SWI/SNF is the prototype chromatin remodeling complex and regulates the expression of 5% genes in yeast. Within SWI/SNF, Snf2 functions as the ATP-dependent motor that drives the fundamental DNA translocation reaction underlying chromatin remodeling, whereas many of the auxiliary subunits target the enzyme to specific loci of the genome. To understand the mechanism of nucleosome recognition, we report the cryo-EM structure of the yeast SWI/SNF complex in complex with the mononucleosome. Based on the specific biological activities involved, the SWI/SNF complex is delineated into three functional modules: the motor module, the actin-related protein (ARP) module, and SRM.

Most of the auxiliary subunits are assembled into the SRM, which is further delineated into two lobes, the DNA-binding lobe (DBL), and the histone-binding lobe (HBL). These auxiliary subunits recognize different features of the DNA and histone components of the nucleosome, and collectively provide the structural basis for chromatin targeting of the complex. DBL of SWI/SNF is composed of multiple elements, including Snf6, the N-termini of Swi1 and Snf5, and Snf12, which directly or indirectly bind to the DNA. The N-termini of Swi1 and Snf5 interact with each other, which may bind to the DNA of nucleosome either through the ARID domain directly, or indirectly through transcription coactivators, providing the structural basis for their cooperation in SWI/SNF targeting. HBL contains two important elements for histone binding, Snf5 and Taf14. A fragment of the C-terminal tail was found, which folded back and sandwiched between Swi3 and Swp82 at the HBL. Intriguingly, at the periphery of the DBL, we identified an IgG-fold domain of Snf12. Because the SWIB domain inserts into the β6–β7 loop, the IgG-fold is barely detectable at the sequence level. Structural comparison indicated that this IgG-fold domain shows a strong analogy to the YEATS domain of TAF14. This YEATS-like domain is ~9 nm away from the exit DNA without any steric hindrance, which would allow binding to transcription factors in a manner similar to the SWIB domain.

> LQDQYKEGIKVVDIDDPDMMVDSFTMPNISHSNIDYQTLLANSDHAKFTIEPGVLPVGIDTHTATDIYQTLIALNLDTTVNDCLDKLLNDECTESTRENALYDYYALQLLPLQKAVRGHVLQFEWHQNSLLTNTHPNFLSKIRNINVQDALLTNQLYKNHELLKLERKKTEAVARLKSMNKSAINQYNRRQDKKNKRLKFGHRLIATHTNLERDEQKRAEKKAKERLQALKANDEEAYIKLLDQTKDTRITHLLRQTNAFLDSLTRAVKDQQKYTKEMIDSHIKEASEEVDDLSMVPKMKDEEYDDDDDNSNVDYYNVAHRIKEDIKKQPSILVGGTLKDYQIKGLQWMVSLFNNHLNGILADEMGLGKTIQTISLLTYLYEMKNIRGPYLVIVPLSTLSNWSSEFAKWAPTLRTISFKGSPNERKAKQAKIRAGEFDVVLTTFEYIIKERALLSKVKWVHMIIDEGHRMKNAQSKLSLTLNTHYHADYRLILTGTPLQNNLPELWALLNFVLPKIFNSVKSFDEWFNTPFANTGGQDKIELSEEETLLVIRRLHKVLRPFLLRRLKKDVEKELPDKVEKVVKCKMSALQQIMYQQMLKYRRLFIGDQNNKKMVGLRGFNNQIMQLKKICNHPFVFEEVEDQINPTRETNDDIWRVAGKFELLDRILPKLKATGHRVLIFFQMTQIMDIMEDFLRYINIKYLRLDGHTKSDERSELLRLFNAPDSEYLCFILSTRAGGLGLNLQTADTVIIFDTDWNPHQDLQAQDRAHRIGQKNEVRILRLITTNSVEEVILERAYKKLDIDGKVIQAGKFDNKSTSEEQEALLRSLLDAEEERRKKRESGVEEEEELKDSEINEILARNDEEMAVLTRMDEDRSKKEEELGVKSRLLEKSELPDIYSRDIGAELKREESESAAVYNGRGARERKTATYNDNMSEEQWLRQFEVSDDEKNDKQARKQRTKKEDKSEAIDGGGSGGHHHHHH;> SNQLISNYAASNSMDRSSSASNEFVPNTSDNNNNSNNHNMRNNSNNKTSNNNNVTAVPAATPANTNNSTSNANTVFSERAAMFAALQQKQQQRFQALQQQQQQQQNQQQQNQQPQQQQQQQQNPKFLQSQRQQQQRSILQSLNPALQEKISTELNNKQYELFMKSLIENCKKRNMPLQSIPEIGNRKINLFYLYMLVQKFGGADQVTRTQQWSMVAQRLQISDYQQLESIYFRILLPYERHMISQEGIKETQAKRIFLQQFLQELLKKVQQQQQAAALANANNNINSASSAPTPAAPGASVPATAAPGTEAGIVPVSANTPKSLNSNININVNNNNIGQQQVKKPRKQRVKKKTKKELELERKEREDFQKRQQKLLEDQQRQQKLLLETKLRQQYEIELKKLPKVYKRSIVRNYKPLINRLKHYNGYDINYISKIGEKIDSNKPIFLFAPELGAINLHALSMSLQSKNLGEINTALNTLLVTSADSNLKISLVKYPELLDSLAILGMNLLSNLSQNVVPYHRNTSDYYYEDAGSNQYYVTQHDKMVDKIFEKVNNNATLTPNDSNDEKVTILVDSLTGNQLPTPTPTEMEPDLDTECFISMQSTSPAVKQWDLLPEPIRFLPNQFPLKIHRTPYLTSLKKIKDEIDDPFTKINTRGAEDPKVLINDQLSTISMILRNISFSDNNSRIMSRNFYLKRFISDLLWLVLIHPENFTCNRKILNFKKDLVIVLSNISHLLEIASSIDCLLILILVISFGQPKLNPMASSSSFGSESLTFNEFQLQWGKYQTFGVDILAKLFSLEKPNLNYFKSILLNKNTGNNLYDRNSNNNHKDKKLLRRLLNLYNDNNKNNNNRHNLLNDVVSFLFSAIPLQQVLSQSADPSLLIDQFSPVISQSLTSILVIVQKILPLSNEVFEISENNSDSNSNNNGNKDSSFNFNKNLPFVWLSSEENIGSGLLKLSEIILNINNSTSKNTLLQQQNYSKVLLPSINISCVQLIKCLVEKSICFENCLNNDPEILKKIASIPNLFPTDLEIFQLFTNPSVDIQIINQYQLLYNLKNDILTNLEGGSGGWSHPQFEKWSHPQFEKWSHPQFEK;> MNNQPQGTNSVPNSIGNIFSNIGTPSFNMAQIPQQLYQSLTPQQLQMIQQRHQQLLRSRLQQQQQQQQQTSPPPQTHQSPPPPPQQSQPIANQSATSTPPPPPAPHNLHPQIGQVPLAPAPINLPPQIAQLPLATQQQVLNKLRQQAIAKNNPQVVNAITVAQQQVQRQIEQQKGQQTAQTQLEQQRQLLVQQQQQQQLRNQIQRQQQQQFRHHVQIQQQQQKQQQQQQQHQQQQQQQQQQQQQQQQQQQQQQQQQQQQQQQQQQQQQGQIPQSQQVPQVRSMSGQPPTNVQPTIGQLPQLPKLNLPKYQTIQYDPPETKLPYPTYWSDKKADTDTLLYEQIIQRDKINKYSLIRETNGYDPFSIYGFSNKEYISRLWHTLKYYQDLKNTRMKSITSTSQKIPSASIWGNGYSGYGNGITNTTTRVIPQVEVGNRKHYLEDKLKVYKQAMNETSEQLVPIRLEFDQDRDRFFLRDTLLWNKNDKLIKIEDFVDDMLRDYRFEDATREQHIDTICQSIQEQIQEFQGNPYIELNQDRLGGDDLRIRIKLDIVVGQNQLIDQFEWDISNSDNCPEEFAESMCQELELPGEFVTAIAHSIREQVHMYHKSLALLGYNFDGSAIEDDDIRSRMLPTITLDDVYRPAAESKIFTPNLLQISAAELERLDKDKDRDTRRKRRQGRSNRRGMLALSGTSASNTSMNGVHNTVAAGNASSLPPGEILLPDIADIPRTFRTPVPSTLMPGGVDVGPSVESYELRNTTTYKSRPDRPKPVSPPCYIIDHIPGHSLLLSIKLPGKVNTKEEFAAAPNDTSSGTNAMLPSPESLKTKLNSNIRAGVTIPSIPNPIANHTVTNSPNPTLQPVIPGGAASKSVPTPSLPIAPPVAPHDSEATLLTNSNNGSSNNNTQNTGGSGGDYKDDDDK;>[2x]MENTLGEGSTVNASVDVDQHGNDNNSDSNANAAVAGVANTDTAGEESQQQDESLKDEATVPNTRDAESEAITVTAKQQPTMQANKLDSQETPSTEESRAQNVFGQDNEDSDNLFGETESSVSNNEANTPSIPTNPVDNENNKPAIKEDSTIQDSNGDVKNMEDVKIQKEEEPENNTVIEGVKEESQPDENTKEMDEVEEDDEDDDQPMISPDNSIFGDTKSESKQLGNTSSVANTPSEIPDAHKAEQEDIIEKTESVDKKVDSGEERNEQEREIMNDHSKSANPKKTTITRVEPETFEIPQAHEIVIPSYSKWFNLEKIHSIEVQSLPEFFTNRIPSKTPEVYMRYRNFMVNSYRLNPNEYFSVTTARRNVSGDAAALFRLHKFLTKWGLINYQVDSKLLPKNIEPPLTSQYSTRHDAPRGLFPFESYKPSVQLPDMAKLKKMMNTSDSESTLYKYLKESKRKYDEITHPPSTTDDENGDKNDNGGKMNNEVSTSTSMTGDANLLEEGETSRPLKKVKILEQIDENWSKEDLQKLLKGIQEFGADWYKVAKNVGNKSPEQCILRFLQLPIEDKFLYGDGNGKGDNDNGLGPLKYAPHLPFSKSENPVLSTIAFLVGLVNPKTVQSMTQRAIQSAESIKSQKEEISDQKPIEHIKEGSEIAISSLGYRSHIFATNEERQMNFLTNELIRLQMEKLDAKLNHLKKLEKFMELERKTLERQQENLLIQRLNFNQNSSKIVNVLSKCLNLISDSNINNSSVAEKEEIRSQIDHFKSMLSKPETLSIGKNPFNKPNIETGENHNGQSISNENDVKPISIEAPQFYRYWSAGGSGGHHHHHH;> MSKVMKPSNGKGSRKSSKAATPDTKNFFHAKKKDPVNQDKANNASQITPTVPHSHPSDMVIPDHLAELIPELYSFQQLVDSEKRLDHFIHLRNLHMKRMVAQWERSKLSQEFLYPHLNFPNVKFLRIFISNVSENQPWQMDTNNEADLMALENATWTMRIEGRLLDNVQANDPAREKFSSFIESIVVDFKNKENDNVPSTKFNAAPEENATEGPSDKKLNLNLPLQFSLPNGDNSTTTNTDQNNATMGEETAKKDMSSTTPKLESVKWQYDPNNPVDFDGLDIKRVGSENVECTISILRKSSPEEPFMSYSPQLTAIIGLKSGTSHDAIFSIYKYIHLNELLTNDESAFENLMGNRNNHNSNTSTSKMLDAASSQVSIVKLDTQLITLLPSSLKESSPDTMKLTDLLSLINSTHLLPLQPIEIDYTVRVDKASTYGELVLDIEVPDVNALKFNNTQRESQIGAAELNENARELEQIKPKIALQDKEITSVLSNLHESNKRYRFFKKISEDPVKALNECIASTSNALKVLSGDEGYNEDMVRRANFYKENEAMLRENIEVILSNGRM;> MGVIKKKRSHHGKASRQQYYSGVQVGGVGSMGAINNNIPSLTSFAEENNYQYGYSGSSAGMNGRSLTYAQQQLNKQRQDFERVRLRPEQLSNIIHDESDTISFRSNLLKNFISSNDAFNMLSLTTVPCDRIEKSRLFSEKTIRYLMQKQHEMKTQAAELQEKPLTPLKYTKLIAAAEDGSRSTKDMIDAVFEQDSHLRYQPDGVVVHRDDPALVGKLRGDLREAPADYWTHAYRDVLAQYHEAKERIRQKEVTAGEAQDEASLQQQQQQDLQQQQQVVTTVASQSPHATATEKEPVPAVVDDPLENMFGDYSNEPFNTNFDDEFGDLDAVFF;> MLGEDEGNTVLEKGNNPSVKQGEVGAVFIVPKILIREHERVILKQILQILDQDELVQPPLDKFPYKKLELPKYIDELKTRDATNTSYKMIQLDAYGEKKVGSNGELFGGRHYLFNTFTFTAHMGVLLVLLQDVIKVLYQSNATHDEDEFIVQHDQILVMETSEEQTKFLAKNGVIPEESKGSFKYITARSAFVEFGASVIAGGQRIVDDYWESLAKKQNLSSHQRVFKLSTNLISKISLLRPSFQNNRISNANEISANTNNTCTISTSKFESQYPIVTEQPSAEIREAYIENFAKGEHISAIVPGQSISGTLELSAQFRVPRYHSKNSFQQALQMKAMDIPIGRHEELLAQYESQAPDGSASISLPNHIPSVNPSNKPIKRMLSSILDINVSSSKNKKSEENEMIKPMNKGQHKNNTSLNINGWKFESLPLKSAENSGKQQYYRGLPLYEKNTLLERLKQLTPNEIKELEHLHDAVFVNTGLQNVRKVRTKKWKKYWQYKAGIPIGLKRSQLDEFKNKYLKDVLAQTSVTTNFNEITNTDETITTKRVPNPNFLGNCNIKDFKPPYIYSHVNKVPQNVAGDKTAVKLDTEVKNTNANPVVATDPVAAKPDNLANFSNEVAMNNGGSGGHHHHHH>RAVDLVDDSNDVDNSIEAEEEKPRNRAFEADWLKFTKTPPTKLQQADGATIEIVCEMMGSQVPSIQWVVGHLPRSELDDLDSNQVAEEAPSAIVRVRSSHIIDHVLSEARTYTCVGRTGSKTIYASTVVHPPRSSRLTPEKTYPGAQKPRIIYTEKTHLDLMGSNIQLPCRVHARPRAEITWLNNENKEIVQGHRHRVLANGDLLISEIKWEDMGNYKCIARNVVGKD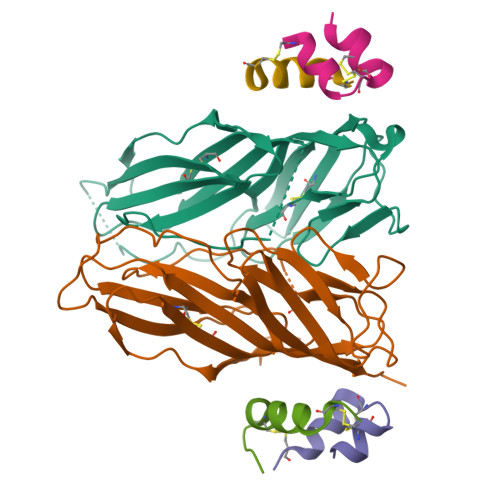TADTFVYPVLNEED[4x];>[4x]DFRGVVDSCCRNSCSFSTLRAYCDS;>[4x]NSLRACGPALMDMLRVACPNGFNSMFAK> XXXXXXXXXXXXXXXXXXXXXXXXXXXXXXXXXXXXXXXXSQNLEEEKKQRNHFKSIQAKILEKYGTHKPESPVLKIVNVTQTSCVLAWDPLKLGSAKLKSLILYRKGIRSMVIPNPFKVTTTKISGLSVDTPYEFQLKLITTSGTLWSEKVILRTH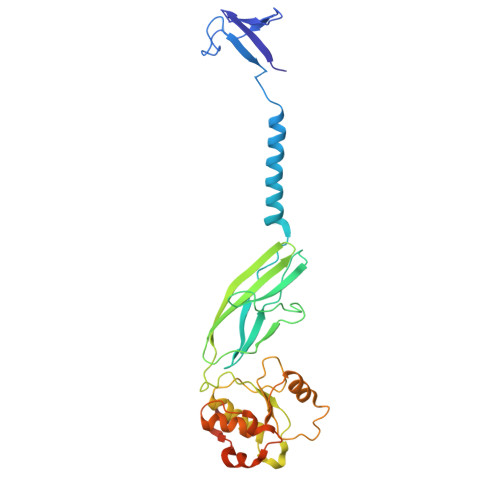KMTDMSGITVCLGPLDPLKEISDLQISQCLSHIGARPLQRHVAIDTTHFVCNDLDNEESNEELIRAKHNNIPIVRPEWVRACEVEKRIVGVRGFYLDADQSILKSYTFPPVNEEELSYSKENEPVAEVADENK>[5x]MGNDISLIALLAFSTLLPFIIASGTCFVKFSIVFVMVRNALGLQQIPSNMTLNGVALLLSMFVMWPIMHDAYVYFEDEDVTFNDISSLSKHVDEGLDGYRDYLI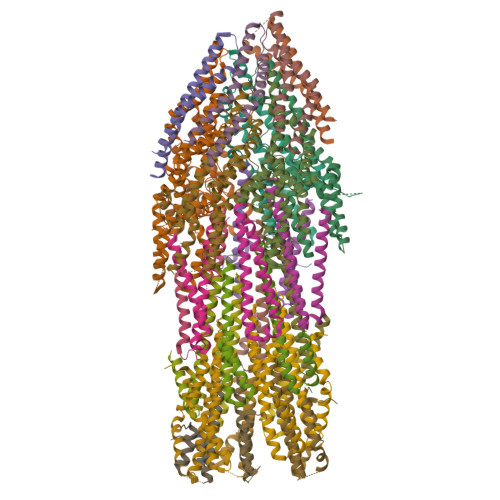KYSDRELVQFFENAQLKRQYGEETETVKRDKDEIEKPSIFALLPAYALSEIKSAFKIGFYLYLPFVVVDLVVSSVLLALGMMMMSPVTISTPIKLVLFVALDGWTLLSKGLILQYMDIAT;> MFYALYFEIHHLVASAALGFARVAPIFFFLPFLNSGVLSGAPRNAIIILVALGVWPHALNEAPPFLSVAMIPLVLQEAAVGVMLGCLLSWPFWVMHALGCIIDNQRGATLSSSIDPANGIDTSEMANFLNMFAAVVYLQNGGLVTMVDVLNKSYQLCDPMNECTPSLPPLLTFINQVAQNALVLASPVVLVLLLSEVFLGLLSRFAPQMNAFAISLTVKSGIAVLIMLLYFSPVLPDNVLRLSFQATGLSSWFYERGATHVLE;>MDDLVFAGNKALYLVLILSGWPTIVATIIGLLVGLFQTVTQLQEQTLPFGIKLLGVCLCLFLLSGWYGEVLLSYGRQVIFLALAKG[4x];>MSIATIVPENAVIGQAVNIRSMETDIVSLDDRLLQAFSGSAIATAVDKQTITNRIEDPNLVTDPKELAISQEMISDYNLYVSMVSTLTRKGVGAVETLLRS[6x];>[17x]MATPWSGYLDDVSAKFDTGVDNLQTQVTEALDKLAAKPSDPALLAAYQSKLSEYNLYRNAQSNTVKVFKDIDAAIIQNFR>[20x]S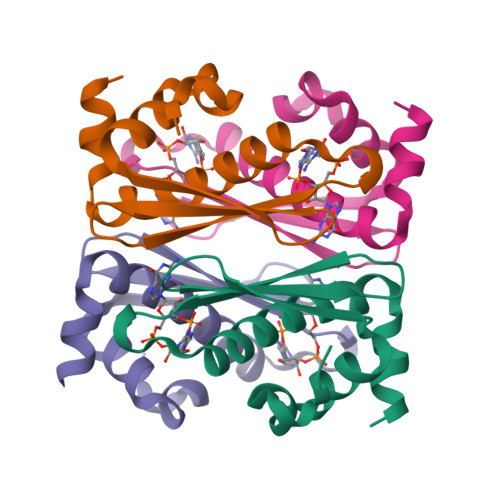MKINAENFECLRESKLKRKVYEDLVKEATFVRVSPKSTVCVVTDHNSFEVIGTSSVYKVENFNDEIGRDTALSQALDSFIKFLAYSGELSDVLENI1-[5-({4-[3-(trifluoromethyl)phenyl]piperazin-1-yl}sulfonyl)-2,3-dihydro-1H-indol-1-yl]ethan-1-one 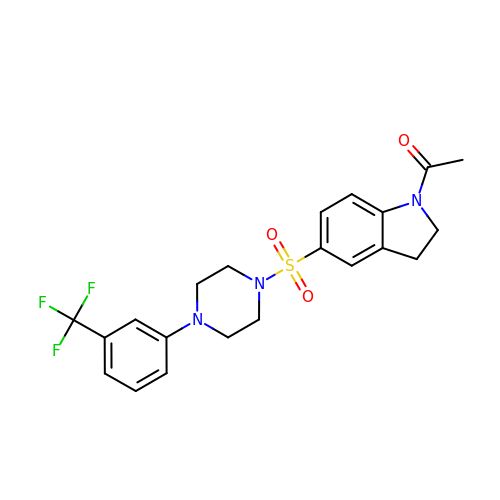| C21 H22 F3 N3 O3 S | JRTCXCIMCOKGMN-UHFFFAOYSA-N>MRYPVTLTPAPEGGYMVSFVDIPEALTQGETVAEAMEAAKDALLTAFDFYFEDNELIPLPSPLNSHDHFI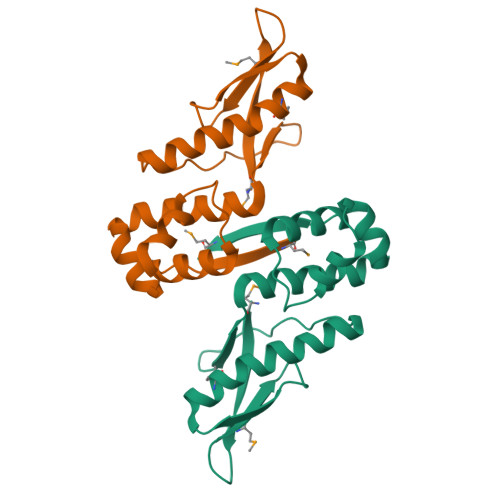EVPLSVASKVLLLNAFLQSEITQQELARRIGKPKQEITRLFNLHHATKIDAVQLAAKALGKELSLVMV[2x]>SNAMGTKNIGKGLTFEDILLVPNYSEVLPREVSLETKLTKNVSLKIPLISSAMDTVTEHLMAVGMARLGGIGIIHKNMDMESQVNEVLKVKNSGGLRVGAAIGVNEIERAKLLVEAGVDVIVLDSAHGHSLNIIRTLKEIKSKMNIDVIVGNVVTEEATKELIENGADGIKVGIGPGSICTTRIVAGVGVPQITAIEKCSSVASKFGIPIIADGGIRYSGDIGKALAVGASSVMIGSILAGTEESPGEKELIGDTVYKYYRGMGSVGAMKSGSGDRYFQEKRPENKMVPEGIEGRVKYKGEMEGVVYQLVGGLRSCMGYLGSASIEELWKKSSYVEITTSGLRESHVHDVEIVKEVMNYSK[4x]

Inosine 5′-monophosphate dehydrogenase (IMPDH) is a promising target for the treatment of Cryptosporidium infections. Adenosine is converted into guanine nucleotides in a process that requires IMP dehydrogenase (IMPDH) activity. IMPDH is a homotetramer with square-planar symmetry. The reduced cofactor dissociates from the enzyme and the mobile active-site flap (residues 302–330) folds into the cofactor site, positioning the catalytic Arg315 to activate water for the hydrolysis of E-XMP* to yield the product xanthosine 5′-monophosphate (XMP).

Here, the structure of C. parvum IMPDH (CpIMPDH) in complex with inosine 5′-monophosphate (IMP) and P131, an inhibitor with in vivo anticryptosporidial activity, is reported. P131 contains two aromatic groups, one of which interacts with the hypoxanthine ring of IMP, while the second interacts with the aromatic ring of a tyrosine in the adjacent subunit. The electron density indicates that Cys219 has oxidized to the sulfenic acid, as often occurs with reactive cysteine residues. The oxime group of P131 lies across the hypoxanthine ring of IMP, while the N5 amine forms hydrogen bonds to the main-chain carbonyl O atom of Gly212 and N3 of IMP in all of the subunits. The amine also interacts with water molecules to create a hydrogen-bonding network that extends to the 2′-OH of IMP, the sulfenic acid of Cys219, Ala165 N, Gly212 O, Gly214 N, Thr221 OG, Asp252 O and Tyr358 OH′. The right-side aromatic ring binds in the adenosine subsite formed by residues Ser22′, Val24′-Leu25′-Pro26′, Ser164-Ala165-His166, Ser354′ and Gly357′-Tyr358′. This subsite is highly divergent, accounting for the selectivity of the CpIMPDH inhibitors. In subunits A, C and D, the NO2 group is roughly parallel to the aromatic ring and forms water-mediated hydrogen bonds to Ser22 O′, Val24 O′, Ser164 OG, His166 O, Ser169 O and Asn171 N and ND2. The water-mediated hydrogen-bonding networks of both the left-side alkylamine and the right-side NO2 group offer many opportunities for further inhibitor optimization.(2R,3S)-heptane-1,2,3-triol | C7 H16 O3 | 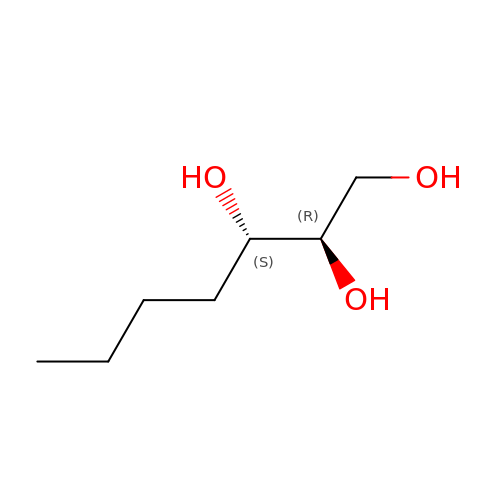HXYCHJFUBNTKQR-NKWVEPMBSA-N>[2x]DALKVNRAPVGVEPQEVHKWLQSFNWDFKENRTKYPTKYHMANETKEQFKVIAKEYARMEAAKDERQFGTLLDGLTRLGAGNKVHPRWGETMKVISNFLEVGEYNAIAASAMLWDSATAAEQKNGYLAQVLDEIRHTHQCAFINHYYSKHYHDPAGHNDARRTRAIGPLWKGMKRVFADGFISGDAVECSVNLQLVGEACFTNPLIVAVTEWASANGDEITPTVFLSVETDELRHMANGYQTVVSIANDPASAKFLNTDLNNAFWTQQKYFTPVLGYLFEYGSKFKVEPWVKTWNRWVYEDWGGIWIGRLGKYGVESPASLRDAKRDAYWAHHDLALAAYAMWPLGFARLALPDEEDQAWFEANYPGWADHYGKIFNEWKKLGYEDPKSGFIPYQWLLANGHDVYIDRVSQVPFIPSLAKGTGSLRVHEFNGKKHSLTDDWGERQWLIEPERYECHNVFEQYEGRELSEVIAEGHGVRSDGKTLIAQPHTRGDNLWTLEDIKRAGCVFPDPLAKF;>[2x]PQSSQVTKRGLTDPERAAIIAAAVPDHALDTQRKYHYFIQPRWKRLSEYEQLSCYAQPNPDWIAGGLDWGDWTQKFHGGRPSWGNESTELRTTDWYRHRDPARRWHHPYVKDKSEEARYTQRFLAAYSSEGSIRTIDPYWRDEILNKYFGALLYSEYGLFNAHSSVGRDCLSDTIRQTAVFAALDKVDNAQMIQMERLFIAKLV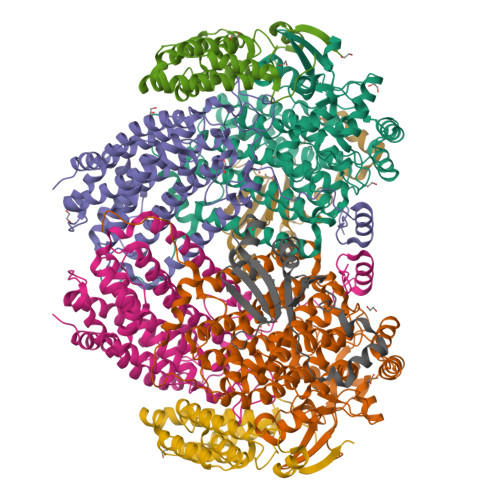PGFDASTDVPKKIWTTDPIYSGARATVQEIWQGVQDWNEILWAGHAVYDATFGQFARREFFQRLATVYGDTLTPFFTAQSQTYFQTTRGAIDDLFVYCLANDSEFGAHNRTFLNAWTEHYLASSVAALKDFVGLYAKVEKVAGATDRAGVSEALQRVFGDWKIDYADKIGFRVDVDQKVDAVLAGYKN;>[2x]AKREPIHDNSIRTEWEAKIAKLTSVDQATKFIQDFRLAYTSPFRKSYDIDVDYQYIERKIEEKLSVLKTEKLPVADLITKATTGEDAAAVEATWIAKIKAAKSKYEAERIHIEFRQLYKPPVLPVNVFLRTDAALGTVLMEIRNTDYYGTPLEGLRKERGVKVLHLQA;>[2x]SAHNAYNAGIMQKTGKAFADEFFAEENQVVHESNAVVLVLMKSDEIDAIIEDIVLKGGKAKNPSIVVEDKAGFWWIKADGAIEIDAAEAGELLGKPFSVYDLLINVASAVGRAYTLGTKFTITSELMGLDR> MRGSHHHHHHLRQCSGKQEWPELVGERGSK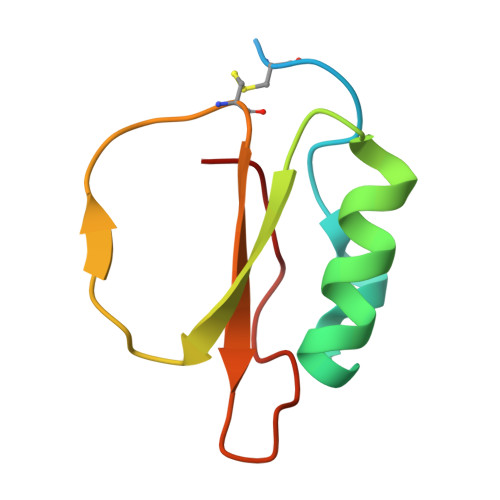AAKIIENENEDVRAIVLPEGSAVPRDLRCDRVWVFVDERGVVVDTPVVM3'-methoxy[1,1'-biphenyl]-4-carboxylic 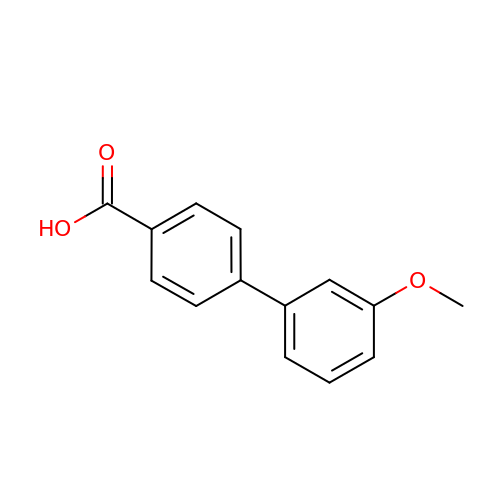acid | C14 H12 O3 | OAMJQKDGQYAQKD-UHFFFAOYSA-N>[2x]GHMNKDNLRSPICCILGHVATGKTKLLDKIRQTNVQEGEA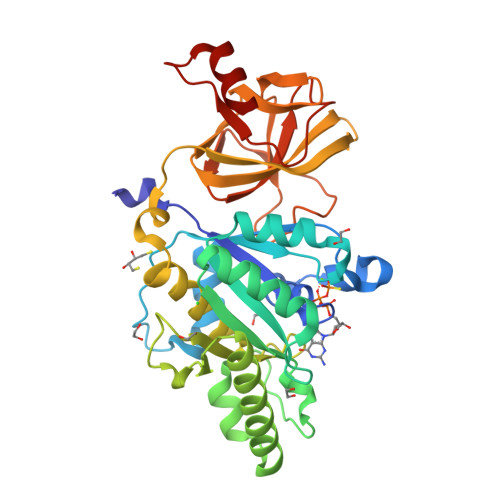GGITQQIGATYFPVEAIKQKTAVVNKDGKFEFKVPGLLIIDTPGHESFSNLRSRGSSLCNIAILVVDIMHGLEPQTIESLRLLRERKTPFVVALNKIDRLYGWKKIENNGFRESFALQNKAVQNEFRNRLDQVKLQFAEQGFNSELFYENKNFARYVSLVPTSAHTGEGIPDMLKLIVQLCQERMASSLMYLSELQATVLEVKAIEGFGVTIDVILSNGILREGDRIVLCGLEGPIKTNIRALLTPAPMRELRIKGQYIHHKEVKAAQGVKISAPGLEGAIAGSRLLVVGPDDDEEELEEEVESD> VTGEEVLQNACAACHVQHEDGRWERIDAARKTPEGWDMTVTRMMRNHGVALEPEERAAIVRHLSDTRGLSLAETEERRYILEREPVAWDEGPDTSMTQTCGRCHSYARVALQRRTPEDWKHLVNFHLGQFPTLEYQALARDRDWWGIAQAEIIPFLARTYPLGEAPDAYADDASGAYVLAGRQPGRGDYTGRLVLKKAGEDYEVTMTLDFADGSRSFSGTGRILGAGEWRATLSDGTVTIRQIFALQDGRFSGRWHDADSDVIGGRLAAVKADAAPQVLAVAPARLKIGEETQLRVAGTGLGSDLTLPEGVAGSVESAGNGVTVLKLTATGTPGPVSLELGGQKVDLVAYDRPDRISIVPDLTIARIGGNGGPIPKVPAQFEAMGWLNGPDGQPGTGDDIALGAFPASWATDNFDEEAEKMQDAKYAGSIDDTGLFTPAEAGPNPERPMQTNNAGNLKVIATVDAEGEPLSAEAHLYATVQRFVDAPIR;> RDYILAPARPDKLVVIDTEKMAVDKVITIADAGPTPMVPMVAPGGRIAYATVNKSESLVKIDLVTGETLGRIDLSTPEERVKSLFGAALSPDGKTLAIYESPVRLELTHFEVQPTRVALYDAETLSRRKAFEAPRQITMLAWARDGSKLYGLGRDLHVMDPEAGTLVEDKPIQSWE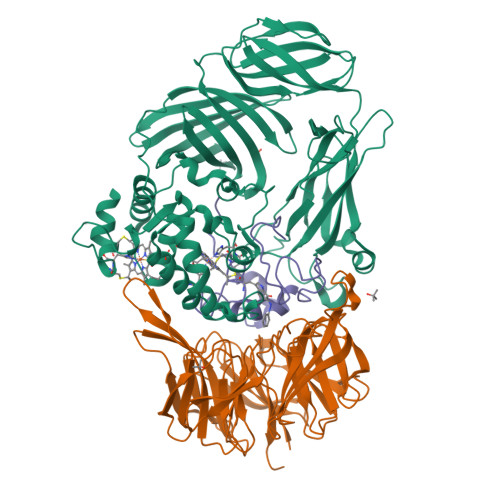AETYAQPDVLAVWNQHESSGVMATPFYTARKDIDPADPTAYRTGLLTMDLETGEMAMREVRIMDVFYFSTAVNPAKTRAFGAYNVLESFDLEKNASIKRVPLPHSYYSVNVSTDGSTVWLGGALGDLAAYDAETLEKKGQVDLPGNASMSLASVRLFTRDE;> MNALVGCTTSFDPGWEVDAFGAVSNLCQPMEADLYGCADPCWWPAQVADTLNTYPNWSAGADDVMQDWRKLQSVFPETK>[2x]GAMAPVASASPKLCLAWQGMLLLKNSNFPSNMHLLQGDLQVASSLLVEGSTGGKVAQLKITQRLRLDQPKLDEVTRRIKVAGPNGYAILLAVPGSSDSRSSSSSAASDTATSTQRPLRNLVSYLKQKQAAGVISLPVGGNKDKENTGVLHAFPPCEFSQQFLDSPAKALAKSEEDYLVMIIVRGFGFQI

The SPOC (Spen orthologue and paralogue C-terminal) domain is a 15–20 kDa protein domain found across eukaryotic species from yeast to mammals. SPOC domains form a distorted β-barrel structure comprising seven β-strands and a variable number of α-helices. SHARP (SMRT/HDAC1 associated repressor protein), RBM15, and RBM15B (RNA binding motif protein 15/15B) paralogues belong to the Spen family of proteins characterized by a series of N-terminal RRMs (RNA recognition motifs) and the C-terminal SPOC domain. Here we show that the SPOC domains of DIDO, SHARP, and RBM15 act as CTD reader domains that bind phosphorylated serines via conserved surface patches.

We solved the crystal structure of RBM15 SPOC (to 1.45 Å resolution), which has a distorted β-barrel fold comparable to previously structurally characterized SPOC domains. The conserved lysine and arginine residues cluster to a basic surface patch similar to that of SHARP SPOC. Although RBM15 SPOC dimers were present in the asymmetric unit, SEC-MALS analysis revealed that RBM15 SPOC forms monomers in solution, which was also the case for other SPOC domains. RBM15 SPOC has a preference for serine-5 phosphorylation but also binds phosphorylated serine-2 and serine-7 with similar affinity. We modeled RBM15 SPOC binding to an 8-mer CTD peptide phosphorylated at serine-5. In the model, phosphorylated serine-5 is tightly coordinated by the conserved residues K795, R834, and K898. Compared to SHARP SPOC, RBM15 SPOC had a clear preference for double phosphorylated CTD peptides and mutation of the highly conserved R834 to alanine reduced, but did not completely abrogate the binding to 2×S5P CTD. This indicates that there might be a second basic patch on the surface of RBM15 SPOC. Indeed, our RBM15 SPOC structure shows a potential second interaction surface at a distance from the conserved basic patch comparable to that between the two patches of PHF3 and DIDO SPOC (patch 2, distance to patch 1: 21 Å). Amino acids R847, R848, and K850 are potential candidates for electrostatic coordination of phosphoserine from the second CTD repeat.YO3-biotin | C21 H19 N2 O | 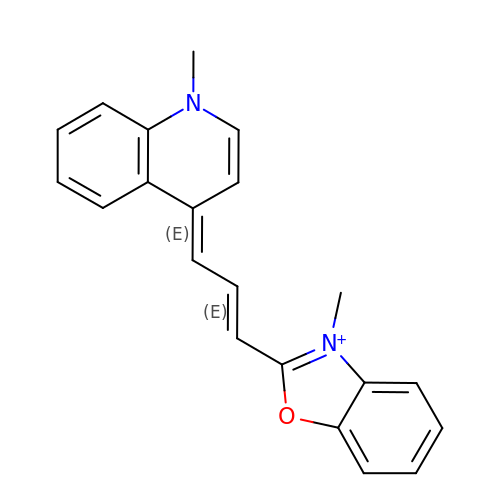VHMUTYCKXYROKA-UHFFFAOYSA-N>MKILSKSIEKMQSDTQEANDIVTLANLQYNGSTPADAFETKVTNIIDRLNNNGIHINNKVACQLIMRGLSGEYKFLRYTRHRHLNMTVAELFLDIHAIYEEQQGSRNPLEHHHHHH[3x]

Excessive replication of Saccharomyces cerevisiae Ty1 retrotransposons is regulated by Copy Number Control, a process requiring the p22/p18 protein produced from a sub-genomic transcript initiated within Ty1 GAG. To minimize genomic damage, p22/p18 interrupts virus-like particle function by interaction with Gag. Thus, p22 is identical to the C-terminal half of Gag-p49 and is processed at the C-terminus by PR to generate a mature protein p18, that is identical to the C-terminal half of mature capsid Gag-p4525,27. The structure comprises an all α-helical domain related to that observed in the CA-CTD of the yeast Ty3 retrotransposon, ARC proteins, and orthoretroviruses.

We determined the crystal structures of p18mAUG1 and p18mAUG2 expressed in E. coli. The p18mAUG1 structure was solved by molecular replacement using the p18mAUG2 structure as a search model. Both constructs crystallised in the same P6522 hexagonal spacegroup with the p18mAUG1 crystals diffracting to a slightly higher resolution of 2.8 Å and the structure refined to an R-factor and Free R-factor of 25.6 and 26.4% respectively. In both structures, the asymmetric unit (ASU) comprises three copies of the p18m monomer. The structure has an all-helical fold making a five-helix bundle (α1-α5) comprising α1 (residues E265-A273), α2 (residues D284-N300), α3 residues (N306-M314), α4 (residues Y321-R330) and α5 (residues V336-Q351). In all copies, residues spanning D262 to Q351 are visible in the electron density map. There is no additional density for residues 249 to 259 that constitute the additional N-terminal sequence difference between AUG1 and AUG2. Quantitative mobility assays revealed that a fragment containing AUG1 to residue 355 of p18 retained potent restriction of Ty1, comparable to full-length p18. In the first (Dimer-1), the exposed surfaces of α1 and α3 pack against α1’ and α3’ of the opposing monomer. In the second interface (Dimer-2), residues on the outer surface of α4 and α5 pack against α4′ and α5′ of the opposing monomer.>MMASAATELDVDGVKVRFTNPDKVYFPKLGKNGTKGKLVEYYLSVASGPMLALLRDRPVHLQRFPDGIEGEEIYQKRVPQKHPDYLETCVVTFPSGRTADALKITHPSSIIWAAQMGTVTLHPWQVRCPDTEHPDELRVDLDPQPGTGFKEARTVACDVLKPLLDELGLVGYPKTSGGRGVHVFLRIKPQWDFIEVRRAGIALAREVERRAPDAVTTSWWKEERGERLFIDYNQNARDRTFASAYSVRKTPIATVSMPLSWDELRNADPDDYTMNTVPDLLAGRDDPWADIDSVQQSLGPLLDLVAADEERGLGDLPYPPNYPKMPGEPPRVQPSKKVAEHWDEQGNRKQ[2x]

Recently, it was reported that a closely related enzyme called Prim–PolC, operonically associated with ligase C (LigC), is specifically involved in LigC-dependent repair of short DNA-gapped intermediates produced during excision-repair processing of lesions in mycobacteria, further expanding the repertoire of pathways in which these diverse replicases operate. A notable feature of Prim–PolC is its favourable activity on short DNA gaps of 1–3 nucleotides, which it preferentially fills in with ribonucleotides. Although the crystal structure of the apo Prim–PolC showed that it is remarkably similar to Prim–PolD, it contains a unique C-terminal extension called Loop 3, proposed to be potentially involved in gap recognition. To understand the molecular basis for its gap-binding and synthesis activities, we elucidated the crystal structures of pre- and post-catalytic intermediates of Prim–PolC bound to DNA substrates containing a two-nucleotide gap.

To understand the molecular basis for substrate recognition and synthesis, we crystallised Prim–PolC (Prim–PolC4–336) in complex with dsDNA containing a two-nucleotide (2-nt) gap. To determine the structure of a pre-catalytic ternary complex of the enzyme bound to the DNA, a non-hydrolysable incoming UTP ribonucleotide (UpNHpp) and manganese ions were also included. Briefly, the elucidated structure shows Prim–PolC bound to a 2-nt gapped DNA substrate in the act of incorporating the appropriate ribonucleotide (UTP) opposite the templating base (A at position 0) in the single-stranded gap. The structure reveals that Prim–PolC contains a conserved phosphate-binding pocket, consisting of N20, K23, Y25, K35 and P65, that engages with the 5′ phosphate on the downstream strand, positioning the N-terminal region of the enzyme on the 5′ side of the gap. Binding of Prim–PolC to DNA induces a major splaying of the template strand by 97.3°. The templating strand sits on Loop 3 and N321 interdigitates into the upstream duplex region, flipping out a guanine base (T/G-2) from the templating strand, and causes it to adopt an extra-helical conformation. N321 appears to act as a molecular locating pin that stops the upstream duplex from slipping back and forth. Residues in Loop 2 contact and support the incoming primer strand, which is docked into the active site of the enzyme, positioning the incoming 3′-OH within the attacking distance of the ribonucleotide analogue (UpNHpp) and metal ions, thus forming a pre-turnover ternary complex. In this ternary complex structure, we observe that the 3′ end of the primer strand adopts a C-3′-endo conformation, and is docked in the active site with the incoming 3′-OH of G-1 positioned only 3.3 Å away from the α-phosphate of the incoming base, and almost in line with the α–β-bond position of the ribonucleotide analogue (UpNHpp).>SMKQYEHVKRDLNPEDFWEIIGELGDGAFGKVYKAQNKETSVLAAAKVIDTKSEEELEDYMVEIDILASCDHPNIVKLLDAFYYENNLWILIEFCAGGAVDAVMLELERPLTESQIQVVCKQTLDALNYLHDNKIIHRDLKAGNILFTLDGDIKLADFGVSAKNTRTIQRRDSFIGTPYWMAPEVVMCETSKDRPYDYKADVWSLGITLIEMAEIEPPHHELNPMRVLLKIAKSEPPTLAQPSRWSSNFKDFLKKCLEKNVDARWTTSQLLQHPFVTVDSNKPIR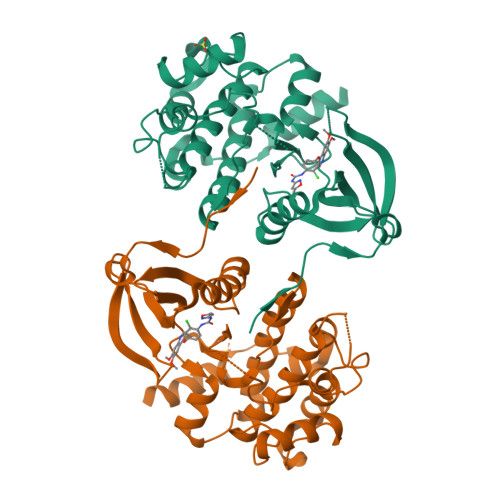ELIAEAKAEVTEEVEDGK[4x]> MKVTVIGAGNVGATVAECVARQDVAKEVVMVDIKDGMPQGKALDMRESSPIHGFDTRVTGTNDYGPTEDSDVCIITAGLPRSPGMSRDDLLAKNTEIVGGVTEQFVEGSPDSTIIVVANPLDVMTYVAYEASGFPTNRVMGMAGVLDTGRFRSFIAEELDVSVRDVQALLMGGHGDTMVPLPRYTTVGGIPVPQLIDDARIEEIVERTKGAGGEIVDLMGTSAWYAPGAAAAEMTEAILKDNKRILPCAAYCD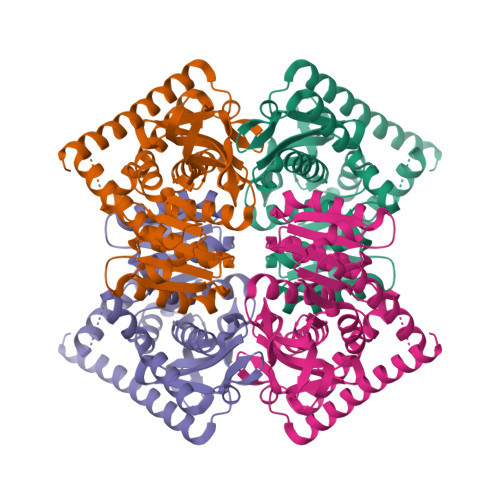GEYGLDDLFIGVPVKLGAGGVEEVIEVDLDADEKAQLKTSAGHVHSNLDDLQRLRDEGKIG>MSEFRIHHDVNELLSLLRVHGGDGAEVYIDLLQKNRTPYVTTTVSAHSAKVKIAEFSRTPEDFLKKYDELKSKNTRNLDPLVYLLSKLTEDKETLQYLQQNAKERAELAAAAVGSSTTSINVPAAASKISMQELEELRKQLGSVATGSTLQQSLELKRKMLRDKQNKKNSGQHLPIFPAWVYERPALIGDFLIGAGISTDTALPIGTLPLASQESAVVEDLLYVLVGVDGRYVSAQPLAGRQSRTFLVDPNLDLSIRELVHRILPVAASYSAVTRFIEEKSSFEYGQVNHALAAAMRTLVKEHLILVSQLEQLHRQGLLSLQKLWFYIQPAMRTMDILASLATSVDKGECLGGSTLSLLHDRSFSYTGDSQAQELCLYLTKAASAPYFEVLEKWIYRGIIHDPYSEFMVEEHELRKERIQEDYNDKYWDQRYTIVQQQIPSFLQKMADKILSTGKYLNVVRECGHDVTCPVAKEIIYTLKERAYVEQIEKAFNYASKVLLDFLMEEKELVAHLRSIKRYFLMDQGDFFVHFMDLAEEELRKPVEDITPPRLEALLELALRMSTANTDPFKDDLKIDLMPHDLITQLLRVLAIETKQEKAMAHADPTELALSGLEAFSFDYIVKWPLSLIINRKALTRYQMLFRHMFYCKHVERQLCSVWISNKTAKQHSLHSAQWFAGAFTLRQRMLNFVQNIQYYMMFEVMEPTWHILEKNLKSASNIDDVLGHHTGFLDTCLKDCMLTNPELLKVFSKLMSVCVMFTNCMQKFTQSMKLDGELGGQTLEHSTVLGLPAGAEERARKELARKHLAEHADTVQLVSGFEATINKFDKNFSAHLLDLLARLSIYSTSDCEHGMASVISRLDFNGFYTERLERLSAERSQKATPQVPVLRGPPAPAPRVAVTAQ[2x];>MATPDQKSPNVLLQNLCCRILGRSEADVAQQFQYAVRVIGSNFAPTVERDEFLVAEKIKKELIRQRREADAALFSELHRKLHSQGVLKNKWSILYLLLSLSEDPRRQPSKVSSYATLFAQALPRDAHSTPYYYARPQTLPLSYQDRSAQSAQSSGSVGSSGISSIGLCALSGPAPAPQSLLPGQSNQAPGVGDCLRQQLGSRLAWTLTANQPSSQATTSKGVPSAVSRNMTRSRREGDTGGTMEITEAALVRDILYVFQGIDGKNIKMNNTENCYKVEGKANLSRSLRDTAVRLSELGWLHNKIRRYTDQRSLDRSFGLVGQSFCAALHQELREYYRLLSVLHSQLQLEDDQGVNLGLESSLTLRRLLVWTYDPKIRLKTLAALVDHCQGRKGGELASAVHAYTKTGDPYMRSLVQHILSLVSHPVLSFLYRWIYDGELEDTYHEFFVASDPTVKTDRLWHDKYTLRKSMIPSFMTMDQSRKVLLIGKSINFLHQVCHDQTPTTKMIAVTKSAESPQDAADLFTDLENAFQGKIDAAYFETSKYLLDVLNKKYSLLDHMQAMRRYLLLGQGDFIRHLMDLLKPELVRPATTLYQHNLTGILETAVRATNAQFDSPEILRRLDVRLLEVSPGDTGWDVFSLDYHVDGPIATVFTRECMSHYLRVFNFLWRAKRMEYILTDIRKGHMCNAKLLRNMPEFSGVLHQCHILASEMVHFIHQMQYYITFEVLECSWDELWNKVQQAQDLDHIIAAHEVFLDTIISRCLLDSDSRALLNQLRAVFDQIIELQNAQDAIYRAALEELQRRLQFEEKKKQREIEGQWGVTAAEEEEENKRIGEFKESIPKMCSQLRILTHFYQGIVQQFLVLLTTSSDESLRFLSFRLDFNEHYKAREPRLRVSLGTRGRRSSHT[4x];>MIHELLLALSGYPGSIFTWNKRSGLQVSQDFPFLHPSETSVLNRLCRLGTDYIRFTEFIEQYTGHVQQQDHHPSQQGQGGLHGIYLRAFCTGLDSVLQPYRQALLDLEQEFLGDPHLSISHVNYFLDQFQLLFPSVMVVVEQIKSQKIHGCQILETVYKHSCGGLPPVRSALEKILAVCHGVMYKQLSAWMLHGLLLDQHEEFFIKQGPSSGNVSAQPEEDEEDLGIGGLTGKQLRELQDLRLIEEENMLAPSLKQFSLRVEILPSYIPVRVAEKILFVGESVQMFENQNVNLTRKGSILKNQEDTFAAELHRLKQQPLFSLVDFEQVVDRIRSTVAEHLWKLMVEESDLLGQLKIIKDFYLLGRGELFQAFIDTAQHMLKTPPTAVTEHDVNVAFQQSAHKVLLDDDNLLPLLHLTIEYHGKEHKADATQAREGPSRETSPREAPASGWAALGLSYKVQWPLHILFTPAVLEKYNVVFKYLLSVRRVQAELQHCWALQMQRKHLKSNQTDAIKWRLRNHMAFLVDNLQYYLQVDVLESQFSQLLHQINSTRDFESIRLAHDHFLSNLLAQSFILLKPVFHCLNEILDLCHSFCSLVSQNLGPLDERGAAQLSILVKGFSRQSSLLFKILSSVRNHQINSDLAQLLLRLDYNKYYTQAGGTLGSFGM[2x];>MARHGPPWSRLDAQQERDVRELVRGVAGLQDEADPNFQLALNFAWSNFRFHRFLDVNSHKIEKTIEGIYEKFVIHSDLSKAASWKRLTEEFLNAPLPSIKEIKTDAHYSILSLLLCLSDSPSNSSYVETPRNKEVEKKDDFDWGKYLMEDEEMDIGPYMDTPNWSEESEEENDQQPLSREDSGIQVDRTPLEEQDQNRKLDPCISWKDEPDDRSWLEHHVVHQYWTARPSQFPHSLHLHSNLAAVWDQHLYSSDPLYVPDDRVLVTETQVIRETLWLLSGVKKLFIFQLIDGKVTVRNNIIVTHLTHSCLRSVLEQIAAYGQVVFRLQEFIDEVMGHSSESMLPGSGSVPKKSTEAPFRTYQAFMWALYKYFISFKEELAEIEKCIINNDTTITLAIVVDKLAPRLSQLKVLHKVFSTGVAEVPPDTRNVVRASHLLNTLYKAILEYDNVGEASEQTVSLLFSLWVETVRPYLQTVDEWIVHGHLWDGAREFIIQRNKNVPVNHRDFWYATYTLYSVSEKTENEEKMSDNASASSGSDQGPSSRQHTMVSFLKPVLKQIIMAGKSMQLLKNLQCAESTTCQAGARDAERKSLYTLFLESVQSRLRHGEDSTPQVLTEQQATKENLMKMQSIAESHLELDDVHDPLLAINFARMYLEQSDFHEKFAGGDVCVDRSSESVTCQTFELTLRSCLYPHIDKQYLDCCGNLMQTLKKDYRLVEYLQAMRNFFLMEGGDTMYDFYTSIFDKIREKETWQNVSFLNVQLQEAVGQRYPEDSSRLSISFENVDTAKKKLPVHILDGLTLSYKVPWPVDIVISLECQKIYNQVFLLLLQIKWAKYSLDVLLFGELVSTAEKPRLKEGLIHEQDTVAQFGPQKEPVRQQIHRMFLLRVKLMHFVNSLHNYIMTRILHSTGLEFQHQVEEAKDLDQLIKIHYRYLSTIHDRCLLREKVSFVKEAIMKVLNLALMFADGWQAGLGTWRMESIEKMESDFKNCHMFLVTILNKAVCRGSFPHLESLALSLMAGMEQS[2x];> MASITQLFDDLCEALLPAAKTHLGQRSVNRKRAKRSLKKVAYNALFTNLFQDETQQLQPDMSKLPARNKILMLSFDLRVGGLGPKADRLEELVEELEAAPCCPLLEVGSVLDLLVQLAGSGPPQVLPRKRDYFLNNKHVGRNVPYSGYDCDDLSVFEMDVQSLISREECLCHSMIQETLQVMEAAPGTGLPTVGLFSFGDPCGDRFERDTRVSLFGALVHSRTYDMDVRLGLPPVPDNADLSGLAIKVPPSVDQWEDEGFQSASNLTPDSQSEPSVTPDVDLWEAALTYEASKRRCWERVGCPPGHREEPYLTEAGRDAFDKFCRLHQGELQLLAGGVLQAPQPVLVKECELVKDVLNVLIGVVSATFSLCQPAQAFVVKRGVHVSGASPESISSLLSEVAEYGTCYTRLSHFSLQPVLDSLYSKGLVFQAFTSGLRRYLQYYRACVLSTPPTLSLLTIGFLFKKLGRQLRYLAELCGVGAVLPGTCGGGPRAAFPTGVKLLSYLYQEALHNCSNEHYPVLLSLLKTSCEPYTRFIHDWVYSGVFRDAYGEFMIQVNHEYLSFRDKLYWTHGYVLISKEVEDCVPVFLKHIAHDIYVCGKTINLLKLCCPRHYLCWSDVPVPRISVIFSLEELKEIEKDCAVYVGRMERVARHSSVSKEEKELRMEIAKQELIAHAREAASRVLSALSDRQMSERMALDARKREQFQRLKEQFVKDQERRQAARQEELDDDFSYARELRDRERRLKSLEEELERKARQALVDHYSKLSAEAARREQKALWRIQRHRLESARLRFLLEDEKHIQEMLKAVSEAHQPQEPPDVLLSVHPQVTSPGPEHPEGGQGCDSGSAEQHSPAWDGWNRPGLLTPQPLKPLAVGAGGRGLQQAEGARPFSDSLSIGDFLPVGPGAEPSVQTGMVPLLEVALQTINLDLPPSAPGEAPAAASTQPSRPQEYDFSTVLRPAVATSPAPGPLQAAECSLGSSGLQLWEDSCGKMDACGSASRETLLPSHPPRRAALEEGSSQPTERLFGQVSGGGLPTGDYASEIAPTRPRWNTHGHVSDASIRVGENVSDVAPTQPRWNTHGHVSNASISLGESVSDVAPTRPRWNIHGHVSNASIRVGENVSDVAPTRPRWNTHGHVSNASIRVGENVSDVAPTRPRWNTHGHVSDASISLGESVSDMAPARPRWNTHGHVSDASISLGESVSDMAPTRPRWNTHGHVSDTSIRVGENVSDVAPIRSRCNTHGHVSDASISLGEPVSDVVSTRPRWNTHVPIPPPHMVLGALSPEAEPNTPRPQQSPPGHTSQSALSLGAQSTVLDCGPRLPVEVGPSLSSPSSGCGEGSISVGENVSDVAPTQPWWPNTPGDSVSEELGPGRSGDTEDLSPNWPLNSQEDTAAQSSPGRGEEAEASAAEAQGGEQAYLAGLAGQYHLERYPDSYESMSEPPIAHLLRPVLPRAFAFPVDPQVQSAADETAVQLSELLTLPVLMKRSITAPLAAHISLVNKAAVDYFFVELHLEAHYEALRHFLLMEDGEFAQSLSDLLFEKLGAGQTPGELLNPLVLNSVLSKALQCSLHGDTPHASNLSLALKYLPEVFAPNAPDVLSCLELRYKVDWPLNIVITEGCVSKYSGVFSFLLQLKLMMWALKDVCFHLKRTALLSHMAGSVQFRQLQLFKHEMQHFVKVIQGYIANQILHVTWCEFRARLATVGDLEEIQRAHAEYLHKAVFRGLLTEKAAPVMNVIHSIFSLVLKFRSQLISQAWGPPGGPRGAEHPNFALMQQSYNTFKYYSHFLFKVVTKLVNRGYQPHLEDFLLRINFNNYYQDA;>[8x]MPREIITLQLGQCGNQIGFEFWKQLCAEHGISPEGIVEEFATEGTDRKDVFFYQADDEHYIPRAVLLDLEPRVIHSILNSPYAKLYNPENIYLSEHGGGAGNNWASGFSQGEKIHEDIFDIIDREADGSDSLEGFVLCHSIAGGTGSGLGSYLLERLNDRYPKKLVQTYSVFPNQDEMSDVVVQPYNSLLTLKRLTQNADCVVVLDNTALNRIATDRLHIQNPSFSQINQLVSTIMSASTTTLRYPGYMNNDLIGLIASLIPTPRLHFLMTGYTPLTTDQSVASVRKTTVLDVMRRLLQPKNVMVSTGRDRQTNHCYIAILNIIQGEVDPTQVHKSLQRIRERKLANFIPWGPASIQVALSRKSPYLPSAHRVSGLMMANHTSISSLFERTCRQYDKLRKREAFLEQFRKEDMFKDNFDEMDTSREIVQQLIDEYHAATRPDYISWGTQEQ;>[3x]MASSSGAGAAAAAAAANLNAVRETMDVLLEISRILNTGLDMETLSICVRLCEQGINPEALSSVIKELRKATEALKAAENMTS

The gamma-tubulin ring complex (γ-TuRC) is the principal microtubule nucleation template in vertebrates. Microtubules are formed de novo in a process termed nucleation, which is spatially and temporally highly controlled by γ-tubulin complexes, composed of γ-tubulin1 and associated γ-tubulin-complex proteins (GCP). In most eukaryotes, microtubules are templated from a preassembled γ-tubulin ring complex (γ-TuRC) that determines the position and direction of microtubule growth. Here, we used cryo-EM to identify and characterize γ-TuRC assembly intermediates after recombinant expression of the complex, which allowed us to delineate a comprehensive stepwise assembly pathway from a stable 6-spoked core to the mature 14-spoked γ-TuRC, identifying successive stabilization and conformational locking of γ-TuSC units as central principles in the assembly process.

On the GCP2(7)-facing side of the 6-spoke assembly, the expansion phase starts with the recruitment of one γ-TuSC unit, forming spokes 5 and 6 of the fully assembled complex. Notably, the conformation of GCPs in this newly recruited γ-TuSC(5,6) unit differs when compared to the fully assembled complex. In particular, the GRIP2 domains and the associated γ-tubulin copies are displaced from their canonical position. Collectively, these data suggest that the recruitment and subsequent ‘conformational locking’ of individual γ-TuSC units assumes a central role during γ-TuRC assembly.S. aureus bone sialoprotein-binding protein (Bbp) is an allelic variant of SdrE. The gene identified from chromosomal DNA isolated from S. aureus subsp. aureusTCH60 encodes bone sialoprotein-binding protein (Bbp) with 1149 amino acids, containing SD-repeats of 154 residues and the ligand-binding A region from 53 to 601 residues further divided into N1, N2 and N3 domains. S. aureus isolated from patients suffering from septic arthritis and osteomyelitis specifically interacts with bone sialoprotein (BSP), a noncollagenous protein of bone and dentine extracellular matrix, mediated by Bbp. As a bifunctional MSCRAMM, Bbp also recognizes the human Fg α chain and inhibits thrombin induced blood coagulation.

Based on sequence alignment of Bbp, SdrG and ClfA, we engineered a plasmid that would generate a recombinant fusion protein covering residues Asn273–Pro598 of Bbp from S. aureus, a segment containing both N2 and N3 domains, with N-terminal GST-tag for purification purposes in Escherichia coli. We obtained apo-Bbp273−598 protein and solved the structure at 2.03 Å resolution, consisting of residues Asn273–Leu584 and additional residues Gly and Ser at N-terminus, two of the remaining five amino acid residues (GPLGS) from digested GST-tag. The apo-Bbp273−598 folds into two distinct domains N2 and N3, both of which have two layers of β-sheets and are structurally similar to the Dev-IgG fold, a variant of IgG fold. The two β-sheets of the N2 domain are composed of A, B and E strands on one side and C, D, D1, F and G strands on the opposite side. In N3 domain, C′, D1′, D2′, F′ and G′ strands form one principal sheet and A′, B′, D′ and E′ strands contribute to the facing sheet. The additional D1′ and D2′ strands present the featured Dev-IgG fold. One difference occurs with regard to the D strand in N2 domain, which parallels with E strand, although exhibiting an antiparallel orientation with the corresponding strand in the description of SdrG, ClfB and ClfA. In the apo-Bbp273−598 structure, the C-terminus with poor electron density extends into the solvent region, thus leading to an open groove. Presumably, a ligand-binding site could exist in the groove.

> GPLGSNNVNDLITVTKQMITEGIKDDGVIQAHDGEHIIYTSDFKIDNAVKAGDTMTVKYDKHTIPSDITDDFTPVDITDPSGEVIAKGTFDLNTKTITYKFTDYVDRYENVNAKLELNSYIDKKEVPNETNLNLTFATADKETSKNVKVEYQKPIVKDESNIQSIFSHLDTTKHEVEQTIYVNPLKLNAKNTNVTIKSGGVADNGDYYTGDGSTIIDSNTEIKVYKVASGQQLPQSNKIYDYSQYEDVTNSVTINKNYGTNMANINFGDIDSAYIVKVVSKYTPGAEDDLAVQQGVRMTTTNKYNYSSYAGYTNTILSTTDSGGGDGTVKP>[8x]YVEGQRKRRNTIHEFKKSAKTTLIKIDPALKIKTKKVNTADQCADRCTRNKGLPFTCK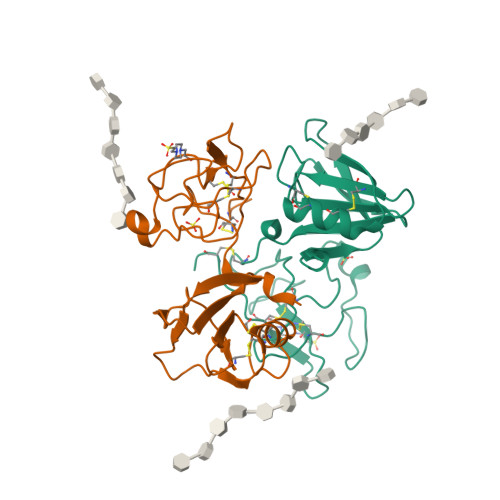AFVFDKARKQCLWFPFNSMSSGVKKEFGHEFDLYENKDYIRNCIIGKGRSYKGTVSITKSGIKCQPWSSMIPHEHSFLPSSYRGKDLQENYCRNPRGEEGGPWCFTSNPEVRYEVCDIPQCSEVE>MVGNPM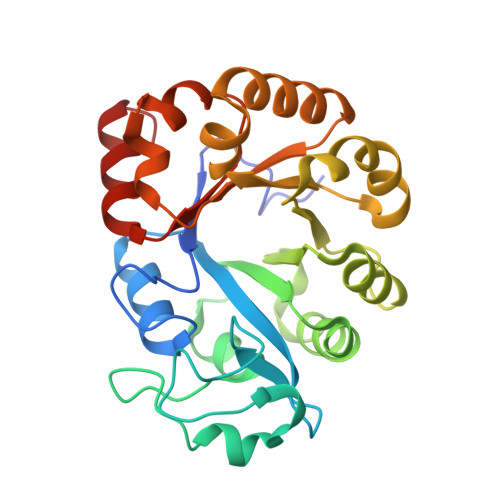WERDKIIVLGHRGYMAKYPENSLLSIRKAIEAGADGVEIDVWLSKDNKVILMHDETIDRTSNLKGRQKEMTLEELKKANIGMGERIPTLEEVFEILPKDALLNIEIKDRDAAKEVARIVSENNPERVMISSFDIEALREYRKYDDTTIMGLLVDKEETVPLIPKLKEKLNLWSVNVPMEAIPIIGFEKTYQAIKWVRSLGLKIVLWTEDDKLFYVDENLKRLLGMFEVVIANDVERMVSYLSSLGIRLE[2x]> MISG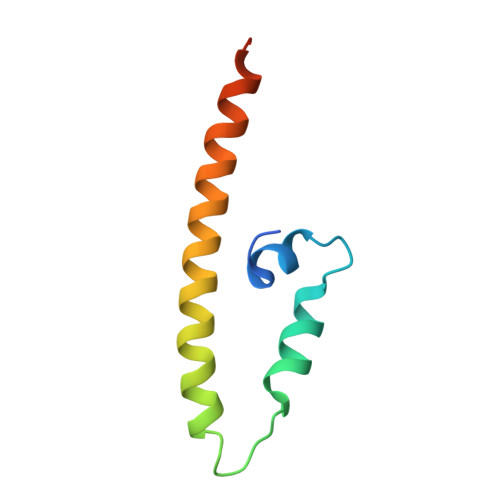ANDPLLDMFFDDDFVPQAFVDILLSSFQTSQLEELKTNCSSLLSKMDYYSGHITKELESTIQVLQKPAELIIY5-(6-oxidanylidene-3~{H}-purin-9-yl)pentylphosphonic acid | C10 H15 N4 O4 P | 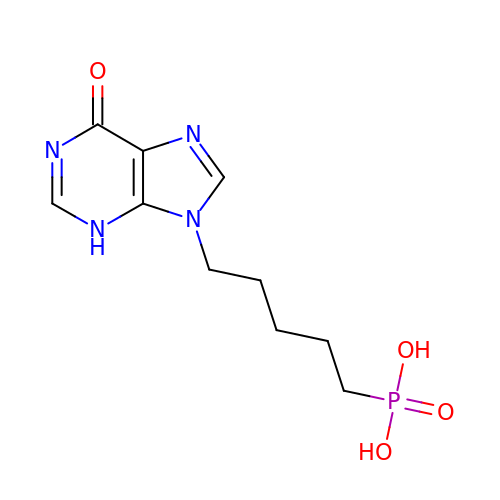HKVZDTLGAPBOBY-UHFFFAOYSA-N> MAQTPAFDKPKVELHVHLDGAIKPETIL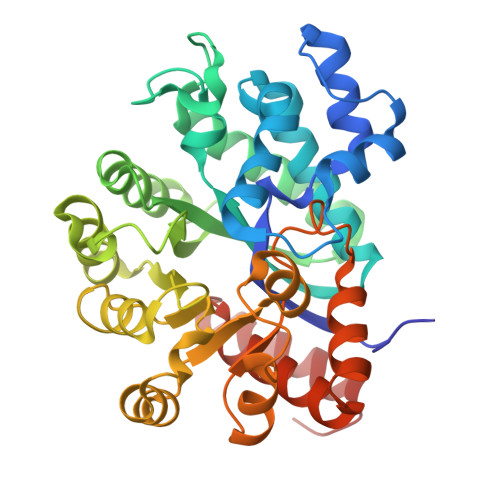YYGKRRGIALPADTPEELLNIIGMDKPLTLPDFLAKFDYYMPAIAGCRDAIKRIAYEFVEMKAKDGVVYVEVRYSPHLLANSKVEPIPWNQAEGDLTPDEVVSLVNQGLQEGERDFGVKVRSILCCMRHQPSWSSEVVELCKKYREQTVVAIDLAGDETIEGSSLFPGHVQAYAEAVKSGVHRTVHAGEVGSANVVKEAVDTLKTERLGHGYHTLEDTTLYNRLRQENMHFEICPWSSYLTGAWKPDTEHAVIRFKNDQVNYSLNTDDPLIFKSTLDTDYQMTKKDMGFTEEEFKRLNINAAKSSFLPEDEKKELLDLLYKAYRMPSPA> MALVYDAEFVGSEREFEEERETFLKGVKAYDGVLATRYLMERSSSAKNDEELLELHQNFILLTGSYACSIDPTEDRYQNVIVRGVNFDERVQRLSTGGSPARYAIVYRRGWRAIAKALDIDEEDVPAIEVRAVKRNPLQPALYRILVRYGRVDLMPVTVDEVPPEMAGEFERLIERYDVPIDEKEERILEILRE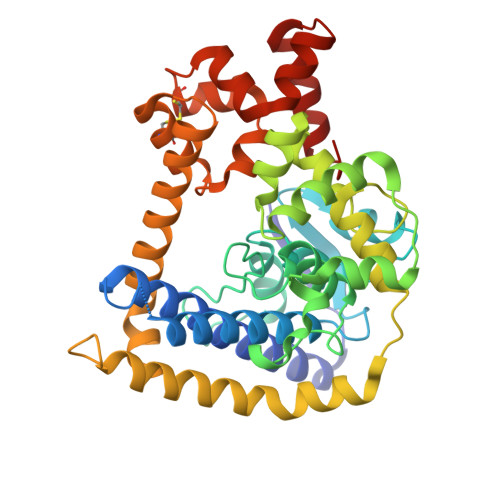NPWTPHDEIARRLGLSVSEVEGEKDPESSGIYSLWSRVVVNIEYDERTAKRHVKRRDRLLEELYEHLEELSERYLRHPLTRRWIVEHKRDIMRRYLEQRIVECALKLQDRYGIREDVALCLARAFDGSISMIATTPYRTLKDVCPDLTLEEAKSVNRTLATLIDEHGLSPDAADELIEHFESIAGI>[2x]TIPSSITSGSIFDLEGDNPNPLVDDSTLVFVPLEA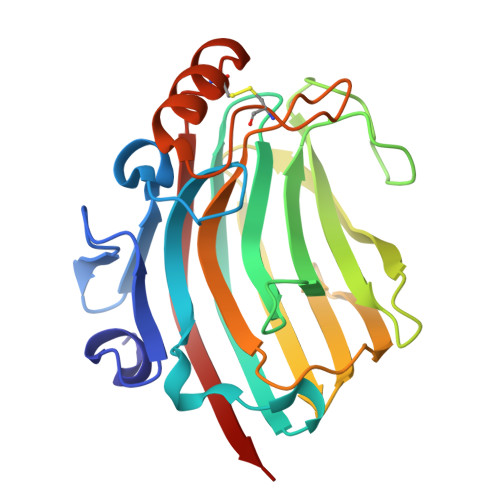QHITPNGNGWRHEYKVKESLRVAMTQTYEVFEATVKVEMSDGGKTIISQHHASDTGTISKVYVSDTDESGFNDSVANNGIFDVYVRLRNTSGNEEKFALGTMTSGETFNLRVVNNYGDVEVTAFGNSFGIPVEDDSQSYFKFGNYLQSQDPYTLDKCGEAGNSNSFKNCFEDLGITESKVTMTNVSYTRETN>[8x]SAAATQAVPAPNQQPEVFCNQIFINNEWHDAVSRKTFPTVNPSTGEVICQVAEGDKEDVDKAVKAARAAFQLGSPWRRMDASHRGRLLNRLADLIERDRTYLAALETLDNGKPYVISYLVDLDMVLKCLRYY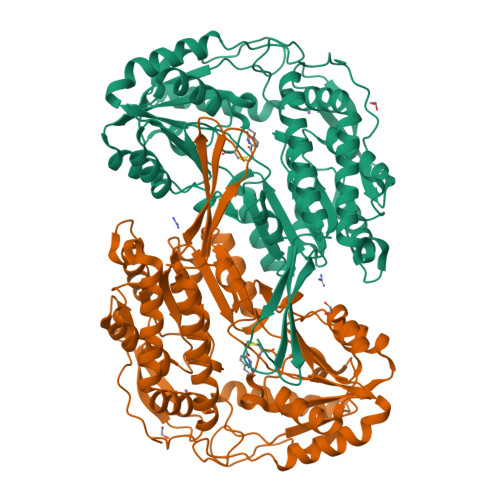AGWADKYHGKTIPIDGDFFSYTRHEPVGVCGQIIPWNFPLLMQAWKLGPALATGNVVVMKVAEQTPLTALYVANLIKEAGFPPGVVNIVPGFGPTAGAAIASHEDVDKVAFTGSTEIGRVIQVAAGSSNLKRVTLELGGKSPNIIMSDADMDWAVEQAHFALFFNQGQCCCAGSRTFVQEDIYDEFVERSVARAKSRVVGNPFDSKTEQGPQVDETQFKKILGYINTGKQEGAKLLCGGGIAADRGYFIQPTVFGDVQDGMTIAKEEIFGPVMQILKFKTIEEVVGRANNSTYGLAAAVFTKDLDKANYLSQALQAGTVWVNCYDVFGAQSPFGGYKMSGSGRELGEYGLQAYTEVKTVTVKVPQKNS>[4x]MMGNNMRKLFSMIANSKDKKEKLIE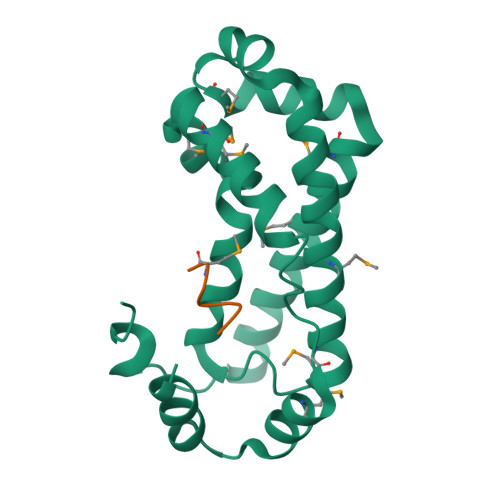SLQENELLNTDEKKKIIDQIKTMHDFFKQMHTNKGALDKVLRNYMKDYRAVIKSIGVDKFKKVYRLLESETMELLHAIAENPNFLFSKFDRSILGIFLPFFSKPIMFKMSIREMDSQIELYGTKLPLLKLFVMTDEEMNFYANLKTIEQYNDYVRDLLMKFDLEKYMEEKGVQNALEHHHHHH>GATESGKRMDCPALPPGWKKEEVIRKSGLSAGKSDVYYFSPSGKKFKSKPQLARYLGNTVDLSSFDFRTGKMMPSKLQK[2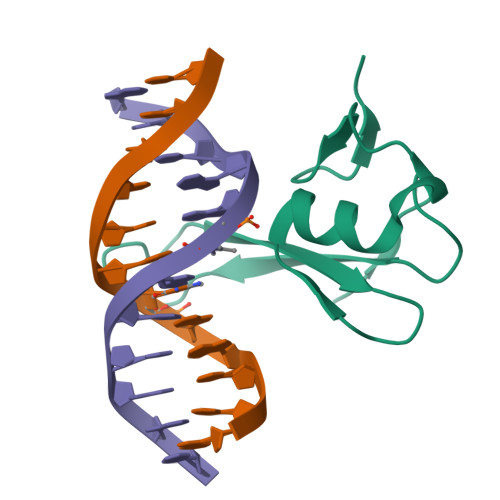x]> VFFSHWTSKYKERNPTEIAYSEDIERIIDSLVTDEITKEEIIHFLFGNFCFHIETMNDQHIADKFKGYQSSCINLKIEPKVDLADLKDHLIQKQQIWESLYGKHLEKIMLRIREKKKKEKEIPDITTAFNQNAAEYEEKYPNCFTNDLSETKTNFSMTWSPSFEKIELSSEVDYNNAIINKFRESFKSSSRVIYNSPYSTNKARDITNLVRLCLTELSCLTRNKNEFCMKETGRENKTIYFKGLAVMNIHMKKLIRHDNEDSLSWCERIKDSLFVLHNGDIREEGKITSVYNNYAKNPECLYIQDSVLKTELETCKKINKLCNDLAIYHYSEDMMQFSKGLMVADRYMTKESFKILTTANTSMMLLAFKSGVPYIALHIVDEDMSDQFNICYTKEIYSYFRNGSNYIYIMRPQRLNQVRLLSLFKTPSKVPVCFAQFSKKANEMEKWLKNKDIEKVNVFSMTMTVKQILINIVFSSVMIGTVTKLSRMGIFDFMRYAGFLPLSDYSNIKEYIRDKFDPDITNVADIYFVNGIKKLLFRMEDLDIIGGITDLNIKCPITGSTLLTLEDLYNNVYLAIYMMPKSLHNHVHNLTSLLNVPAEWELKFRKELGFNIFEDIYPKKAMFDDKDLFSINGALNVKALSDYYLGNIENVGLMRSEIENKEDFLSPCYKISTLKSSKKCSQSNIISTDEIIECLQNAKIQDIENWKGNNLAIIKGLIRTYNEEKNRLVEFFEDNCVNSLYLVEKLKEIINSGSITVGKSVTSKFIRNNHPLTVETYLKTKLYYRNNVTVLKSKKVSEELYDLVKQFHNMMEIDLDSVMNLGKGTEGKKHTFLQMLEFVMSKAKNVTGSVDFLVSVYLMSMKVKMMLYFIEHTFKHVAQSDPSEAISISGDNKIRALSTLSLDTITSYNDILNKNSKKSRLAFLSADQSKWSASDLTYKYVLAIILNPILTTGEASLMIECILMYVKLKKVCIPTDIFLNLRKAQGTFGQNETAIGLLTKGLTTNTYPVSMNWLQGNLNYLSSVYHSCAMKAYHKTLECYKDCDFQTRWIVHSDDNATSLIA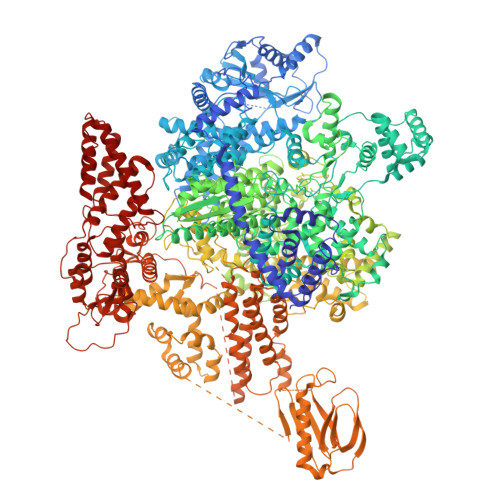SGEVDKMLTDFSSSSLPEMLFRSIEAHFKSFCITLNPKKSYASSSEVEFISERIVNGAIIPLYCRHLANCCTESSHISYFDDLMSLSIHVTMLLRKGCPNEVIPFAYGAVQVQALSIYSMLPGEVNDSIRIFKKLGVSLKSNEIPTNMGGWLTSPIEPLSILGPSSNDQIIYYNVIRDFLNKKSLEEVKDSVSSSSYLQMRFRELKGKYEKGTLEEKDKKMIFLINLFEKATMLTQIIKLPNFINENALNKMSSYKDFSKLYPNLKKNIASSLEMESVHDIMIKNPETILIAPLNDRDFLLSQLFMYTSPSKRNQLSNQSTEKLALDRVLRSKARTKMTYEENMEKKILEMLKFDLDSYCSFKTCVNLVIKDVNFSMLIPILDSAYPCESRKRDNYNFRWFQTEKWIPVVEGSPGLVVMHAVYGSNYIENLGLKNIPLTDDSINVLTSTFGTGLIMEDYCSFKTCVNLVIKDVNFSMLIPILDSAYPCESRKRDNYNFRWFQTEKWIPVVEGSPGLVVMHAVYGSNYIENLGLKNIPLTDDSINVLTSTFGTGLIMEDVKSLVKGKDSFETEAFSNSNECQRLVKACNYMIAAQNRLLAINTCFTRKSFPFYSKFNLGRGFISNTLALLSTIYSKEESYHFVSTASYKLDKTIRTVVSAQQDMNLEKILDTAVYISDKLQSLFPTITREDIVLILQNVCLDSKPIWQSLEDKMKKINNSTASGFTVSNVILSHNSELNTIQKQIVWMWNMGLCSHRTLDFVIRYIRRRDVRYVKTEEQDESGNYVSGTMYKIGIMTRSCYVELIASDQDVAVSLRTPFEILNEREYLFDTYRESIEKLLAEIMFDKVNIINQTTTDCFLRTRRSCIRMTTDNKMIVKVNATSRQIRLENVKLVVKIKYENVDVWDIIESQKSTIKTIKNRLMTSLTFIEAFGNLSQQIKEIVDDDIRETMDEFLMNIRDTCLEGLENCKSVEEYDSYLDENGFNDTVELFENLLRTHDNFENEYSPLFSEIVDKAKQYTRDLEGFKEILLMLKYSLINDASKSYRATGMHAVELMAKKHIEIGEFNLLGMIQLIKACETCHNNDSILNLASLRNVLSRTYATFGRRIRLDHDLDLQNNLMEKSYDFKTLVLPEIKLSELSREILKENGFVISGENLKMDRSDEEFVGLASFNVLRLDEEEMYEGLIKEMKIKRKKKGFLFPANTLLLSELIKFLIGGIKGTSFDIETLLRNSFRPDIFSTDRLGRLSSSVPALKVYATVYMEYKNVNCPLNEIADSLEGYLKLTKSRSKEHFLSGRVKKALIQLRDEQSRTKKLEVYKDIANFLARHPLCLSEKTLYGRYTYSDINDYIMQTREIILSKISELDEVVETDEDNFLLSYL[(2R)-2-methylpiperidin-1-yl](pyrazin-2-yl)methanone 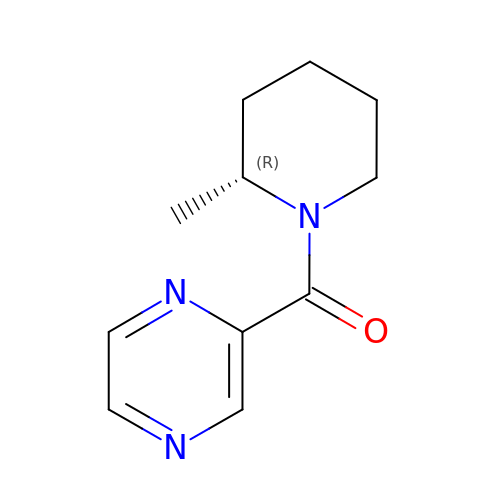| C11 H15 N3 O | MICBEIYHPVLFTJ-SECBINFHSA-N> MARQNLKSTDRAVQQMLDKAKREGIQTVWDRYEAMKPQCGFGETGLCCRHCLQGPCRINPFGDEPKVGICGATAEVIVARGLDRSIAAGAAGHSGHAKHLAHTLKKAVQGKAASYMIKDRTKLHSIAKRLGIPTEGQKDEDIALEVAKAALADFHEKDTPVLWVTTVLPPSRVKVLSAHGLIPAGIDHEIAEIMHRTSMGCDADAQNLLLGGLRCSLADLAGCYMGTDLADILFGTPAPVVTESNLGVLKADAVNVAVHGHNPVLSDIIVSVSKEMENEARAAGATGINVVGICCTGNEVLMRHGIPACTHSVSQEMAMITGALDAMILDYQCIQPSVA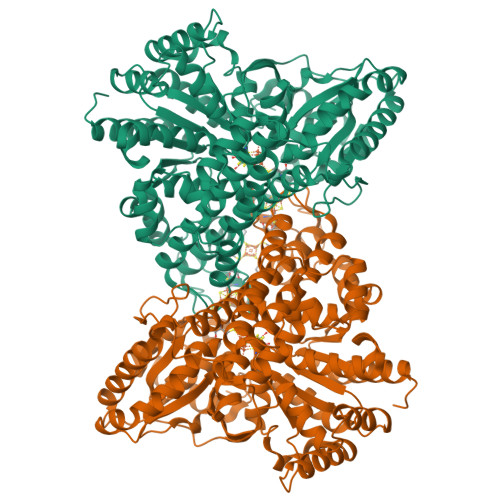TIAECTGTTVITTMEMSKITGATHVNFAEEAAVENAKQILRLAIDTFKRRKGKPVEIPNIKTKVVAGFSTEAIINALSKLNANDPLKPLIDNVVNGNIRGVCLFAGCNNVKVPQDQNFTTIARKLLKQNVLVVATGCGAGALMRHGFMDPANVDELCGDGLKAVLTAIGEANGLGGPLPPVLHMGSCVDNSRAVALVAALANRLGVDLDRLPVVASAAEAMHEKAVAAGTWAVTIGLPTHIGVLPPITGSLPVTQILTSSVKDITGGYFIVELDPETAADKLLAAINERRAGLGLPW> ASNEEDRYLMLSGLQHFQFCKRQWALIHIEQQWEENVRTIEGQHLHKKADQPFMKEKRGSKLTVRAMPIQSKNLQISGICDVVEFVQDSEGIELSGVSGSYKAFPVEYKRGKPKKGDEDIVQLVAQAMCLEEMLVCRIDKGYLFYNEIKHRVEVPITD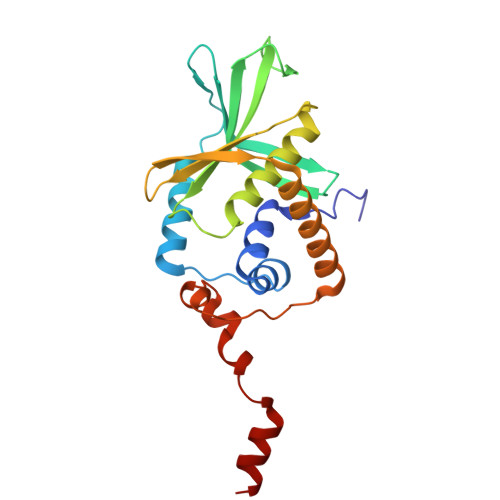ALRDKVVQMAKEMHHYYENRHTPKVKTGPFCNNCSLQSICLPKLMNKRSVKRYIEGRLSE>[2x]TGHPYYLRSFLVVLKTVLENEDDMLLFDEQEKGIVTKFYQLSATGQKLYVRLFQRKLSWIK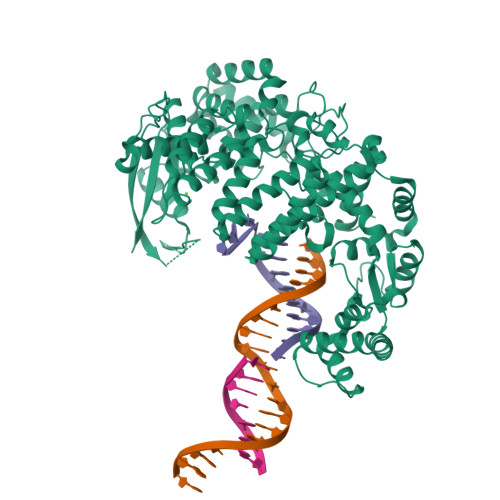MTKLEYEEIALDLTPVIEELTNAGFLQTESELQELSEVLELLSAPELKSLAKTFHLVNPNGQKQQLVDAFLKLAKQRSVIGAVILKRAKALAGQSVRICKGPRAVFSRILLLFSLTDSMEDEDAACGGQGQLSTVLLVNLGRMEFPSYTINRKTHIFQDRDDLIRYAAATHMLSDISSAMANGNWEEAKELAQCAKRDWNRLKNHPSLRCHEDLPLFLRCFTVGWIYTRILSRFVEILQRLHMYEEAVRELESLLSQRIYCPDSRGRWWDRLALNLHQHLKRLEPTIKCITEGLADPEVRTGHRLSLYQRAVRLRESPSCKKFKHLFQQLPEMAVQDVKHVTITGRLCPQRGMCKSVFVMEAGEAADPTTVLCSVEELALAHYRRSGFDQGIHGEGSTFSTLYGLLLWDIIFMDGIPDVFRNACQAFPLDLCTDSFFTSRRPALEARLQLIHDAPEESLRAWVAATWHEQEGRVASLVSWDRFTSLQQAQDLVSCLGGPVLSGVCRHLAADFRHCRGGLPDLVVWNSQSRHFKLVEVKGPNDRLSHKQMIWLAELQKLGAEVEVCHVVAV CA forms the capsid shell surrounding the viral core that protects and transports the viral genome and also interacts with host cell factors that are necessary for trafficking, nuclear entry and proviral integration. Further, we assemble particles from HML2 CArec in vitro and use single-particle cryogenic electron microscopy (cryo-EM) to determine the high-resolution structures of four different types of Fullerene shell assemblies. Our studies of HML2 CArec show that an ERV retains the ability to form capsid assemblies using the same architecture as exogenous viruses. Analysis of the shell structures reveals the intra- and inter-molecular interactions that drives CA assembly into pentamers and hexamers and their association into shells that encapsidate the retroviral genome.

To guide the structural interpretation of these particles at higher resolution, we determined the 1.8 Å crystal structure of the CArec N-terminal domain (CArec-NTD) and the solution NMR structure of CArec C-terminal domain (CArec-CTD). CArec-NTD has the same N-terminal β-hairpin and six-helix fold observed in exogenous orthoretroviral CA proteins. Structural superimposition with exogenous retroviral CA domains revealed the strongest similarity of CArec-NTD with the CA-NTD of the beta and alpharetroviruses Jaagsiekte sheep retrovirus (JSRV) and Rous sarcoma virus (RSV) (Z-scores 10.7 and 9.0) and the most distant relationship to the CA-NTD of the gammaretrovirus MLV. Importantly, although α11 displays the sequential and medium-range inter-residue nuclear Overhauser effect (NOE) cross-peaks that define a helical conformation, the higher T2, lower T1 and lower heteronuclear 1H-15N NOE values observed in NMR relaxation experiments together indicate it is more dynamic than the core domain (α7–α10). These high-resolution structures could be docked directly into the cryo-EM density and, with the additional building of the NTD–CTD linkers, the NTD–CTD interface and helix α8 at the CTD–CTD interface, refined well into each particle structure. Exceptions were the N-terminal β-hairpin that contains a large loop insertion and is more mobile than in the crystal structure, and the NTD–CTD linker region of D5 and D6 equatorial hexamers that displayed weaker density.

>[2x]MPVTLEPMPPGEGAQEGEPPTVEARYKSFSIKMLKDMKEGVKQYGPNSPYMRTLLDSIAHGHRLIPYDWEILAKSSLSPSQFLQFKTWWIDGVQEQVRRNRAANPPVNIDADQLLGIGQNWSTISQQALMQNEAIEQVRAICLRAWEKIQDPLEHHHHHH> GLGYGSWEIDPKDLTFLKELGTGQFGVVKYGKWRGQYDVAIKMIKEGSMSEDEFIEEAKVMMNLSHEKL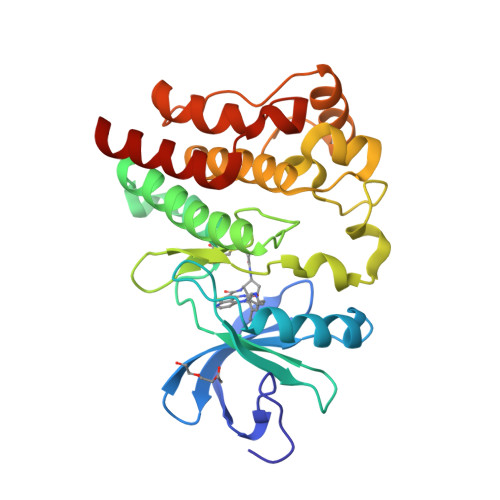VQLYGVCTKQRPIFIITEYMANGCLLNYLREMRHRFQTQQLLEMCKDVCEAMEYLESKQFLHRDLAARNCLVNDQGVVKVSDFGLSRYVLDDEYTSSVGSKFPVRWSPPEVLMYSKFSSKSDIWAFGVLMWEIYSLGKMPYERFTNSETAEHIAQGLRLYRPHLASEKVYTIMYSCWHEKADERPTFKILLSNILDVMDEES>[4x]MRVLVRDLKAHVGQEVELLGFLHWRRDLGRIQFLLLRDRSGVVQVVTGGLKLPLPESALRVRGLVVENAKAPGGLEVQAKEVEVLSPALEPTPVEIPKEEWRANPDTLLEYRYVTLRGEKARAPLKVQAALVRGFRRYLDRQDFTEIFTPKVVRAGAEGGSGLFGVDYFEKRAYLAQSPQLYKQIMVGVFERVYEVAPVWRMEEHHTSRHLNEYLSLDVEMGFIADEEDLMRLEEALLAEMLEEALNTAGDEIRLLGATWPSFPQDIPRLTHAEAKRILKEELGYPVGQDLSEEAERLLGEYAKERWGSDWLFVTRYPRSVRPFYTYPEEDGTTRSFDLLFRGLEITSGGQRIHRYEELLESLKAKGMDPEAFHGYLEVFKYGMPPHGGFAIGAERLTQKLLGLPNVRYARAFPRDRHRLTP;>[2x]MLAHEIRARVARGEVSPLEVAQAYLKRVQELDPGLGAFLSLNERLLEEAEAVDPGLPLAGLVVAVKDNIATRGLRTTAGSRLLENFVPPYEATAVARLKALGALVLGKTNLDEFGMGSSTEHSAFFPTKNPFDPDRVPGGSSGGSAAALAADLAPLALGSDTGGSVRQPAAFCGVYGLKPTYGRVSRFGLIAYASSLDQIGPMARSVRDLALLMDAAAGPDPLDATSLDLPPRFQEALEGPLPPLRLGVVREALAGNSPGVERALEEALKVFRELGLSVREVSWPSLPQALAAYYILAPAEASSNLARYDGTLYGRRAAGEEVEGMMEATRALFGLEVKRRVLVGTFVLSSGYYEAYYGRAQAF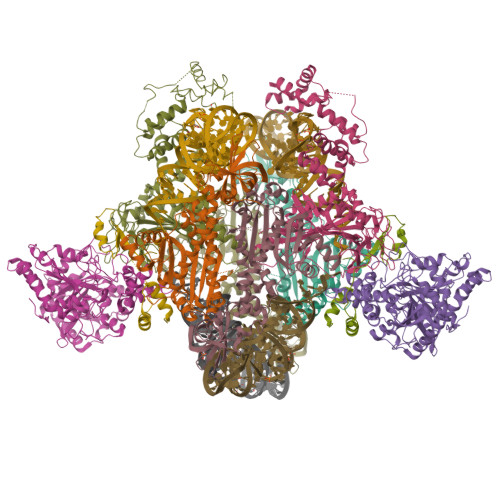RRRLKAEAQALFREVDLLLLPTTPHPAFPFGARRDPLAMYREDLYTVGANLTGLPALSFPAGFEGHLPVGLQLLAPWGEDERLLRAALAFEEATARAHLKAPLGEAL;>MYEAVIGLEVHLHLKTRTKMFCGCRADYFGAEPNTHTCPVCLGLPGALPVPNRVAVEHGLRLALALGAEVPERLVFHRKNYFYPDLPKNYQISQYDLPLGRGGSLPLGERRVRIKRLHLEEDAGKSLHLEGRTLLDLNRAGSPLIELVTEPDLKTPEEARLFLQRIQALVQTLGISDASPEEGKLRADVNVSVRRVGEPLGTKVEIKNLNSFKSVQRALEYEIRRQTEILRRGEKVKQATMGFEEGSGKTYPMRTKEEEADYRYFPEPDLPPVAIPRDWLEEVRRSLPELPWEKEARYRALGIKEKDAEVLAYTPSLARFLDQALPLGLASPQALANWLLADVAGLLHERGLRLEETRLSPEGLARLVGLFERGEVTSRVAKSLLPEVLEGQDPEAXXXXXXXXXXXXXXXXXXXXXXXXXXXXXXXXXXXXXXXXXXXXXXXXXXXXXXXXXXXXXXXXXXXXXX[2x];>MPGMELSPELLRKLETLAKIRLSPEEEALLLQDLKRILDFVDALPRVEEGGAEEALGRLREDEPRPSLPQAEALALAPEAEDGFFRVPPVLE[2x]Structural studies have also illustrated a large conformational change in the G5 loop of the intracellular Ras-type GTPase domain (NFeoB) of the prokaryotic iron transporter FeoB, when comparing crystal structures of apo and nucleotide bound states. The G5 motif is generally comprised of six amino acids with a relatively poor sequence conservation, although the motif invariably forms a loop with electrostatic or hydrophobic interactions with the guanine nucleotide base. We have used the EcNFeoB (Escherichia coli FeoB) protein as a model system because of its clearly resolved conformational change in the G5 loop as revealed by crystal structure analyses. We systematically mutated the residues in the loop to alanine and characterized their biochemical properties in order to determine their individual roles in nucleotide affinity, GTP hydrolysis and GDP release.

Our studies reveal that the intrinsic GDP release rate is highly influenced by the sequence composition of the loop, with the third residue (T151) in particular having an important role in nucleotide affinity. Given their drastic biochemical deviations, we also validated the integrity of the S150A and T151A mutants by determining their crystal structures, which illustrated that the mutations did not have any adverse effects on the overall fold of the protein or on the G5 loop. All other mutants were determined to have slower hydrolysis rates than the wild-type protein, with the T151A mutant being approximately four times slower than the wild-type protein (kcat=0.12 min−1). The most drastic biochemical changes were observed for the T151A mutant protein. Interestingly, the release rate of the T151A mutant was too rapid (>1,000 s−1) to be reliably determined using stopped-flow fluorescence techniques. A threonine residue is also found at this position in many Gα proteins where it coordinates the nucleotide base in an identical way. These stabilizing interactions are abolished in the T151A mutant, resulting in a ~4-fold decreased GDP affinity (Kd=33 μM) and a GDP release rate too rapid to be reliably measured using stopped flow methods (>1000 s−1). Indeed, the stopped-flow fluorescence data indicate that mGDP is spontaneously released even before the competing nucleotide is added to the reaction. The data also indicate a weaker affinity for GMPPNP, which is further supported by the reduced hydrolysis rate. These drastic effects were unexpected given the lack of sequence conservation at this position, although it is notable that the residue at this position is, as far as we know, never found as an alanine or glycine residue.

>[6x]MKKLTIGLIGNPNSGKTTLFNQLTGSRQRVGNWAGVTVERKEGQFSTTDHQVTLVDLPGTYSLTTISSQTSLDEQIACHYILSGDADLLINVVDASNLERNLYLTLQLLELGIPCIVALNMLDIAEKQNIRIEIDALSARLGCPVIPLVSARGRGIEALKLAIDRYKANENVELVHYAQPLLNEADSLAKVMPSDIPLKQRRWLGLQMLEGDIYSRAYAGEASQHLDAALARLRNEMDDPALHIADARYQCIAAICDVVSNTLTAEPSRF>[4x]MSSQFIFEDVPQRNAATFNPEVGYVAFIGKYGQQLNFG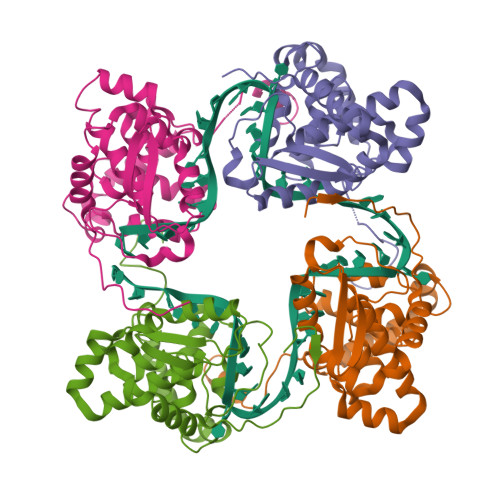VARVFFLNQKKAKMVLHKTAQPSVDLTFGGVKFTVVNNHFPQYVSNPVPDNAITLHRMSGYLARWIADTCKASVLKLAEASAQIVMPLAEVKGCTWADGYTMYLGFAPGAEMFLDAFDFYPLVIEMHRVLKDNMDVNFMKKVLRQRYGTMTAEEWMTQKITEIKAAFNSVGQLAWAKSGFSPAARTFLQQFGINI>[2x]MKKGHHHHHHGSERTGTQPLGVQGLTEEQRMMIRELMDAQMKTFDTTFSHFKNFRLPGVLSSGCELPESLQAPSREEAAKWSQVRKDLCSLKVSLQLRGEDGSVWNYKPPADSGGKEIFSLLPHMADMSTYMFKGIISFAKVISYFRDLPIEDQISLLKGAAFELCQLRFNTVFNAETGTWECGRLSYCLEDTAGGFQQLLLE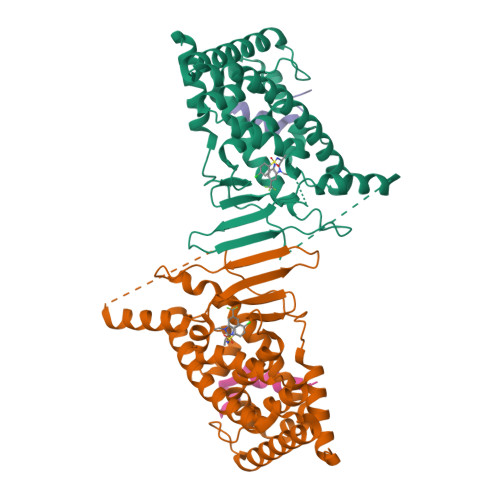PMLKFHYMLKKLQLHEEEYVLMQAISLFSPDRPGVLQHRVVDQLQEQFAITLKSYIECNRPQPAHRFLFLKIMAMLTELRSINAQHTQRLLRIQDIHPFATPLMQELFGIT;>[2x]SLTERHKILHRLLQEGS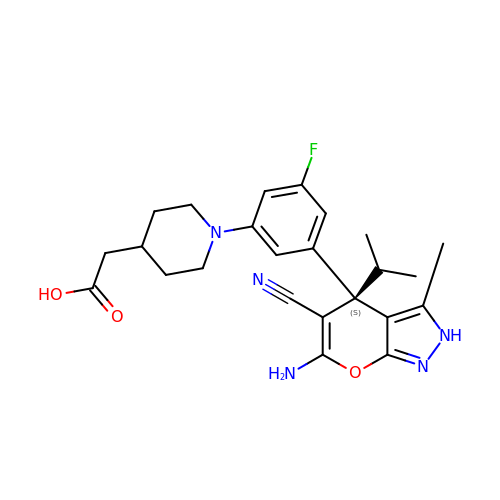2-[1-[3-[(4~{S})-6-azanyl-5-cyano-3-methyl-4-propan-2-yl-2~{H}-pyrano[2,3-c]pyrazol-4-yl]-5-fluoranyl-phenyl]piperidin-4-yl]ethanoic acid | C24 H28 F N5 O3 | LNTOYLXMWSSXMA-DEOSSOPVSA-N>[24x]PKPYVAINMAELKNEPKTFEMFASVGPKVCMVTARHPGFVGFQNHIQIGILPFGNRYGGAKMDMTKESSTVRVLQYTFWKDWKDHEEMHRQNWSYLFRLCYSCASQMIWGPWEPIYEIIYANMPINTEMTDFTAVVGK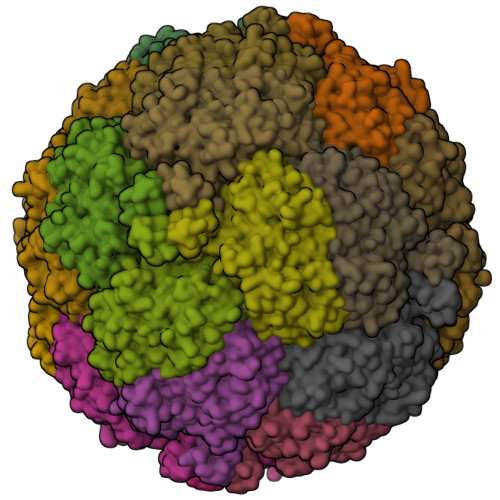KFAEGKPLDIPVISQPYGKRVVAFAEHSVIPGKEKQFEDAIVRTLEMLKKAPGFLGAMVLKEIGVSGIGSMQFGAKGFHQVLENPGSLEPDPNNVMYSVPEAKNTPQQYIVHVEWANTDALMFGMGRVLLYPELRQVHDEVLDTLVYGPYIRILNPMMEGTFWREYLNE> MAAEGYGAASPATATTQDGAKGAAPPNPAASINSPAPAANPEKLTPAQLKAKAKAEKQARRAAAKEAKSAVAAAGQPAQQSGSAGADSKGAAKGKGKQEGQQVPPKGVLVHRPSVSGRRPSIMVVEKDARSGIPECFSHIPMAKRIPTSQAHKDVHPAVLAVGQQMATFALKDSISRLKATLLAFRKVIESYETPKGNSLSRHFVPHVLNPQIEYLTECRPMCFAMGNAIRLLKAKVNKFDINTPEDEAKEGLLEWIDFLINERITLAEYVIARNAAQSINDGDTIVTYGRHRLVEKTLLRARKEGKSFNVTVLDDPYVGEGKELAKVLRHAGIPVLYSPNLGGLRSKV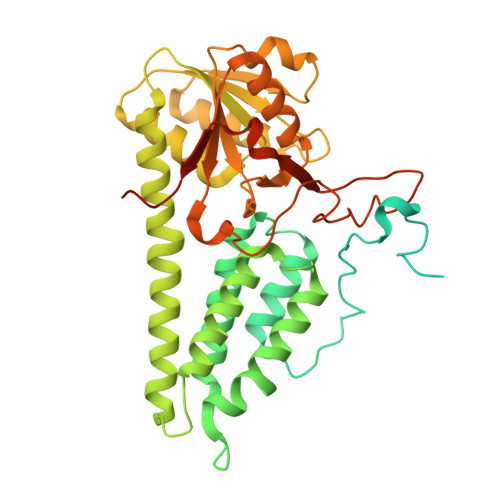PAASNVFLGGEAIFANGSLHAPSGTADVAMAATNAGAKVIVLCETINFDRERVSVDALTYNEIDPERNTGDCFRLLFDNTHERYITGVITEIEFGGGNSPAQAILALLRKQEDPLIA5-acetamido-2,6-anhydro-4-carbamimidamido-3,4,5-trideoxy-7-O-[(2-methoxyethyl)carbamoyl]-D-glycero-D-galacto-non-2-enon ic acid | C16 H27 N5 O9 | 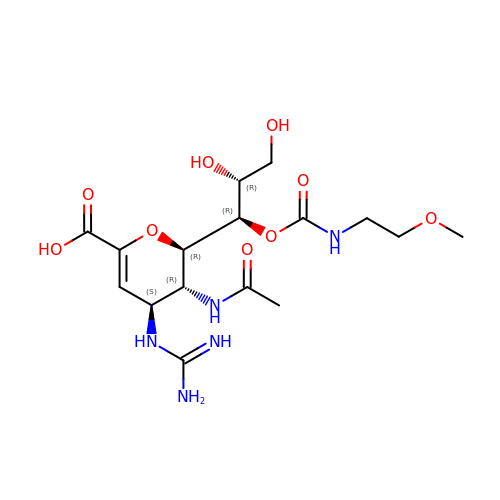VAIHIAVLWLNYQQ-IINAIABHSA-N>MASMTGGQQMGRGSMAGVLPAHGTQHGIRLPLRSGLGGAPLGLRLPRETDEEPEEPGRRGSFVEMVDNLRGKSGQGYYVEMTVGSPPQTLNILVDTGSSNFAV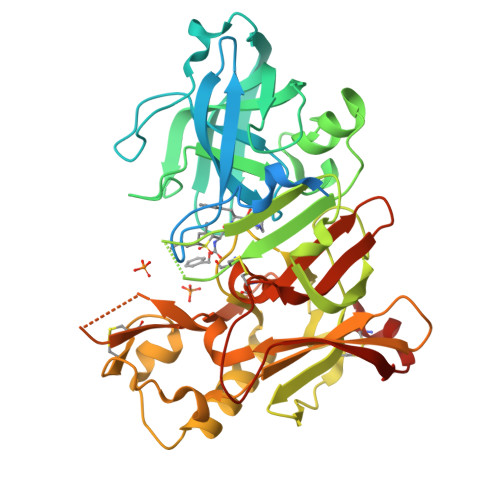GAAPHPFLHRYYQRQLSSTYRDLRKGVYVPYTQGKWEGELGTDLVSIPHGPNVTVRANIAAITESDKFFINGSNWEGILGLAYAEIARPDDSLEPFFDSLVKQTHVPNLFSLQLCGAGFPLNQSEVLASVGGSMIIGGIDHSLYTGSLWYTPIRREWYYEVIIVRVEINGQDLKMDCKEYNYDKSIVDSGTTNLRLPKKVFEAAVKSIKAASSTEKFPDGFWLGEQLVCWQAGTTPWNIFPVISLYLMGEVTNQSFRITILPQQYLRPVEDVATSQDDCYKFAISQSSTGTVMGAVIMEGFYVVFDRARKRIGFAVSACHVHDEFRTAAVEGPFVTLDMEDCGYNIPQTDES[3x]> GSARENE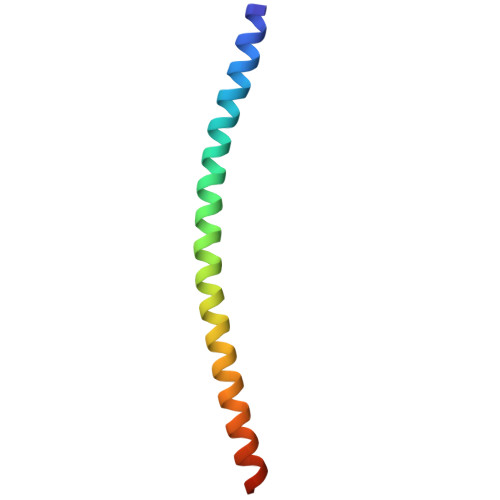MDENLEQVSGIIGNLRHMALDMGNEIDTQNRQIDRIMEKADSNKTRIDEANQRATKML>[2x]GHMEGLAGYVYKAASEGKVLTLAALLLNRSESDIRYLLGYVSQQGGQRSTPLIIAARNGHAKVVRLLLEHYRVQTQQTGTVRFDGYVIDGATALWCAAGAGHFEVVKLLVSHGANVNHTTVTNSTPLRAACFDGRLDIVKYLVENNANISIANKYDNTCLMIAAYKGHTDVVRYLLEQRADPNA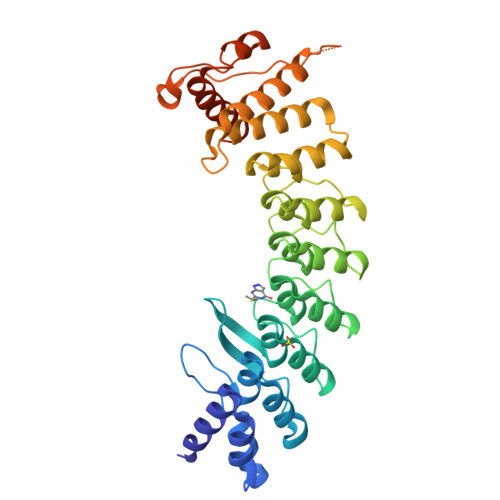KAHCGATALHFAAEAGHIDIVKELIKWRAAIVVNGHGMTPLKVAAESCKADVVELLLSHADCDRRSRIEALELLGASFANDRENYDIIKTYHYLYLAMLERFQDGDNILEKEVLPPIHAYGNRTECRNPQELESIRQDRDALHMEGLIVRERILGGGGSGGGSKKRLLLGLDR> MTQSQTVTVDQQEILNRANEVEAPMADPPTDVPITPCELTAAKNAAQQLVLSADNMREYLAAGAKERQRLATSLRNAAKAYGEVDEEAATALDNDGEGTVQAESAGAVGGDSSAELTDTPRVATAGEPNFMDLKEAARKLETGDQGASLAHFADGWNTFNLTLQGDVKRFRGFDNWEGDAATACEASLDQQRQWILHMAKLSAAMAKQAQYVAQLHVWARREHPTYEDIVGLERLYAENPSARDQILPVYAEYQQRSEKVLTEYNNKAALEPVNPPKPPPAIKIDPPPPPQEQGLIPGFL;> GDALRLARRIAAALNASDNNAGDYGFFWITAVTTDGSIVVANSYGLAYIPDGMEL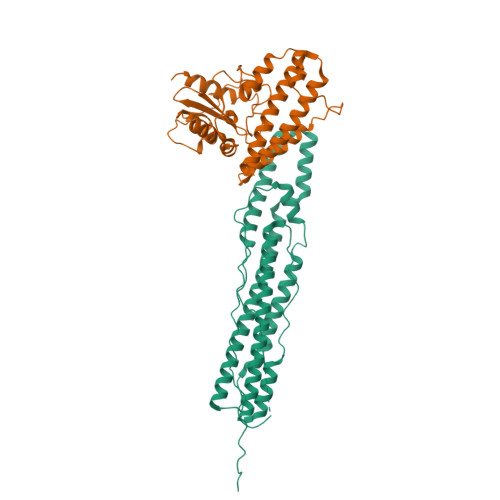PNKVYLASADHAIPVDEIARCATYPVLAVQAWAAFHDMTLRAVIGTAEQLASSDPGVAKIVLEPDDIPESGKMTGRSRLEVVDPSAAAQLADTTDQRLLDLLPPAPVDVNPPGDERHMLWFELMKPMTSTATGREAAHLRAFRAYAAHSQEIALHQAHTATDAAVQRVAVADWLYWQYVTGLLDRALAAAC> MRMFRITACVPSQTRIRTQRELQNTY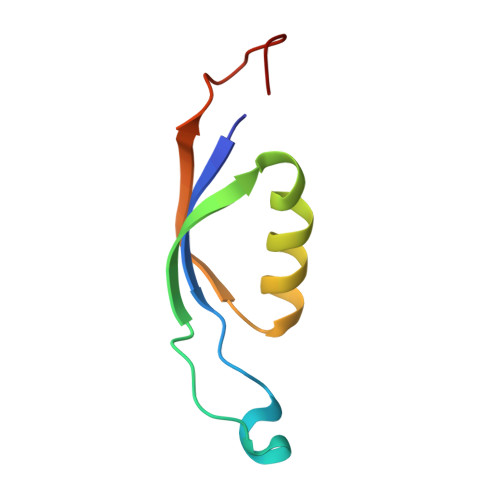FTKLVPYDNWFREQQRIMKMGGKIVKVELATGRPGTNAGLA>HMDDISQDNFLLSKEYENSLDVDTKKASGIYYTPKIIVDYIVKKTLKNHDIIKNPYPRILDISCGCGNFLLEVYDILYDLFEENIYELKKKYDENYWTVDNIHRHILNYCIYGADIDEKAISILKDSLTNKKVVNDLDESDIKINLFCCDSLKKKWRYKFDYIVGNPPYIGHKKLEKKYKKFLLEKYSEVYKDKADLYFCFYKKIIDILKQGGIGSVITPRYFLESLSGKDLREYIKSNVNVQEIVDFLGANIFKNIGVSSCILTFDKKKTKETYIDVFKIKNEDICINKFETLEELLKSSKFEHFNINQRLLSDEWILVNKDDETFYNKIQEKCKYSLEDIAISFQGIITGCDKAFILSKDDVKLNLVDDKFLKCWIKSKNINKYIVDKSEYRLIYSNDIDNENTNKRILDEIIGLYKTKLENRRECKSGIRKWYELQWGREKLFFERKKIMYPYKSNENRFAIDYDNNFSSADVYSFFIKEEYLDKFSYEYLVGILNSSVYDKYFKITAKKMSKNIYDYYPNKVMKIRIFRDNNYEEIENLSKQIISILLNKSIDKGKVEKLQIKMDNLIMDSLGI[3x]

The newly discovered CamA enzyme (named for Clostridioides difficile adenine methyltransferase A) is another orphan MTase, is present in all C. difficile genomes sequenced to date (>300), and is active in all C. difficile genomes subjected to PacBio single-molecule real-time DNA sequencing (which can detect N6-methyladenine—N6mA), but is rarely found in other bacteria. CamA-mediated methylation at CAAAAA (underlining indicates the target A) is required for normal sporulation and biofilm production by C. difficile, a key step in the disease transmission, as well as for colonization in animal models. CamA comprises an N-terminal catalytic domain (residues 1–320) and C-terminal target recognition domain (TRD; residues 320–577). The basic surface of the cleft between the two domains forms the DNA binding site with residues from both domains approaching DNA from opposite directions.

Accordingly, we purified CamA-DNA complexes and grew co-crystals, using a 13-base pair duplex containing a centrally-located A:T and with a 5′-overhang at each end (either an A or T). The complex crystallized in space group P212121, resulting in a structure determined to a resolution of 2.68 Å. In the crystallographic asymmetric unit, there are three CamA-DNA complexes (A, B and C). Thus, the three DNA segments form a pseudo-continuous dsDNA molecule, with two target A residues located on the same strand, while the third target A is located on the opposite strand, in a way representing the presence of methylated CAAAAA on both sense and antisense strands in the genomes of C. difficile isolates. The first 26 residues are disordered in the current structure. Here we describe the interaction of C. difficile CamA with its cognate DNA substrate, resulting in a rearranged A5:T6 base pair immediately 5′ to the flipped-out target adenine (A6). The shifted A5:T6 base pair stacks against the 3′ G7:C7 base pair, as if the target A6 was being squeezed out. Intriguingly, in the CamA-DNA cocrystal structure, we did not observe a bound cofactor in the SAM binding pocket next to the active-site, even though exogenous SAH was added during initial complex formation. However, the added SAH had dissociated during subsequent complex purification, probably due to the low binding affinity.> PISPIETVPVKLKPGMDGPKVKQWPLTEEKIKALVEICTEMEKEGKISKIGPENPYNTPVFAIKKKDSTKWRKLVDFRELNKRTQDFWEVQLGIPHPAGLKKKKSVTVLDVGDAYFSVPLDEDFRKYTAFTIPSINNETPGIRYQYNVLPQGWKGSPAIFQSSMTKILEPFRKQNPDIVIYQYMDDLYVGSDLEIGQHRTKIEELRQHLLRWGLTTPDKKHQKEPPFLWMGYELHPDKWTVQPIVLPEKDSWTVNDICKLVGKLNWASQIYPGIKVRQLSKLLRGTKALTEVIPLTEEAELELAENREILKEPVHGVYYDPSKDLIAEIQKQGQGQWTYQIYQEPFKNLKTGKYARMRGAHTNDVKQLTEAVQKITTESIVIWGKTPKFKLPIQKETWETWWTEYWQATWIPEWEFVNTPPLVKLWYQLEKEPIVGAETFYVDGAANRETKLGKAGYVTNRGRQKVVT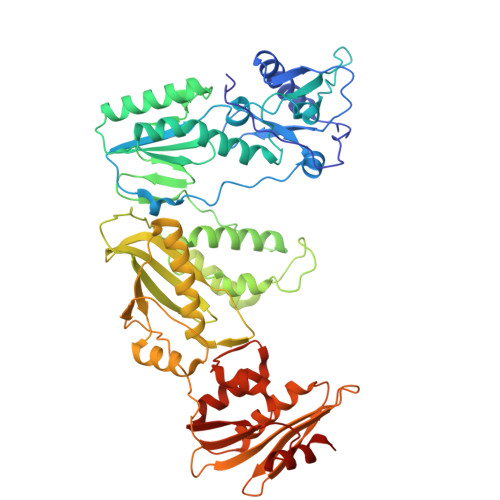LTDTTNQKTELQAIYLALQDSGLEVNIVTDSQYALGIIQAQPDQSESELVNQIIEQLIKKEKVYLAWVPAHKGIGGNEQVDKLVSAGIRK>MASMTGGQQMGRDPNSMKGEIRLIPYEVKANVMEAKETPESIQEIKAPELWSSGFKGKGITIAVLDTGCDTEHPDLKDQIIGGKNFTDDDDGDAENVKDYNGHGTHVAGTIAATDQNGGILGVAPEAKLLIVKVLGGENGSGKYEWIIDGINYAAEQKVDIISMSLGGPSNEPALQEAIQNAVKSGVLVVCAAGNEGDGDE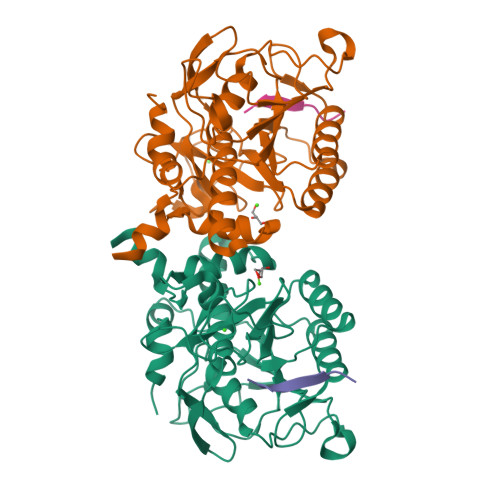RTEEFSYPAAYNEVIAVGSVSLARESSEFSNANKEIDLVAPGEDILSTLPNHKYGRLTGTSMAAPHVSGALAIIKNAEEEAFQRKLTEPEIYAQLVRRTLPLKQSKALVGNGFLYLTAPDVLLEKTLEADLLSLLEHHHHHH[4x]> TVAYIAIGSNLASPLEQVNAALKALGDIPESHILTVSSFYRTPPLGPQDAPDYLNAAVALETSLAPEELLNHTQRIELQQGRVRKAERWGPRTLDLDIMLFGNEVINTERLTVPHYDMKNRGFMLWPLFEIAPELV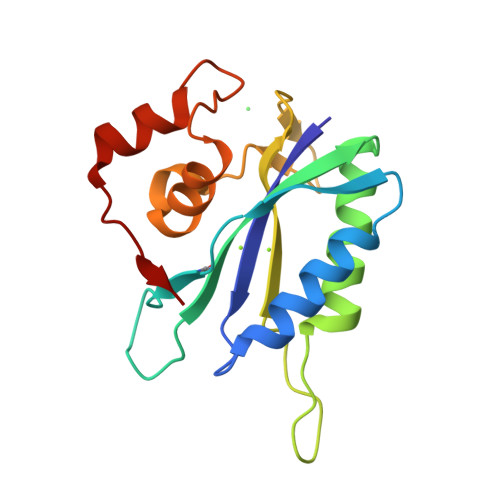FPDGEMLRQILHTRAFDKLNKW Here, we present biochemical and structural evidence that POA inhibits Mtb PanD in a competitive fashion and that it binds with a high degree of complementarity to the active site of the enzyme. PanD is a proenzyme and in the structure, we observed the processed active enzyme after cleavage between Gly24 and Ser25, and modification of Ser25 to a pyruvoyl group (Pyr25). The active protein consists of a β chain (Met1-Gly24) and an α chain (Pyr25 to ILE115). Our results show that resistance to PZA in PanD mutants primarily comes from alterations in two loops covering the active site that have subtle, but significant effects on the affinity and residence time of POA on the enzyme rather than from directly affecting POA binding interactions.

We found that POA also bound to the M117I protein with significantly lower affinity compared to the wild type. The Kd was ~200 µM higher for the mutant than the wild type (Kd = 0.90 (0.09) mM, n = 4; Fig. 3a). We crystallized and solved the structure of the M117I mutant protein. PanD M117I crystallized in the I422 space group and diffracted to 2.33 Å resolution. The structure was very similar to the wild-type protein structure with a root-mean-square difference in the cα positions of 0.32 Å. The crystallization condition contained tartrate, a known inhibitor of the enzyme. A molecule of tartrate fit well into electron density in the active site that could not be accounted for by the protein. In the mutant structure, we could fit an additional 11 residues at C-terminus that were not visible in electron density map for the wild-type protein. The ordered C-terminus enabled us to map several additional resistant mutation sites onto the structure, including M117, that were not visible in the wild-type structure. While none of the mutations were in amino acids that directly contacted POA, most were either on the C-terminal loops of the α and β chain or directly interacting with residues from these loops.

> MLRTMLKSKIHRATVTCADLHYVG;> XVTIDADLMDAADLLEGEQVTIVDIDNGARLVTYAITGERGSGVIGINGAAAHLVHPGDLVILIAYATMDDARARTYQPRIVFVDAYNKPIDIGHDPAFVPENAGELLDPRLGVGLEHHHHHH>MSIKEMPFITCDEFNGVPSYMKSRLTYNQINDVIKEINKAVISKYKILHQPKKSMNSVTRNLYHRFIDEETKDTKGRYFIVEADIKEFTTLKADKKFHVLLNILRHCRRLSEVRGGGLTRYVIT[2x]

Originally discovered in a proteomics screen, the Ska complex is now recognized as a key element required for maintaining stable KT–MT attachments. The ternary Ska complex, composed of Ska1, Ska2 and Ska3, localizes to the outer KT in a KMN-dependent manner. Although GST–Ska1133–255 is not strictly equivalent to the FL Ska1 dimer in the native complex, and thus might bind MTs differently, it clearly interacted with MTs more efficiently than Ska1133–255. These observations suggest that Ska1133–255 (from now on referred to as MTBD) is the major MT-binding element within the Ska complex, which, on dimerization, can bind MTs more efficiently. Here we have used biochemical and high-resolution structural analysis to show that the human Ska complex interacts with MTs through the C-terminal domain of Ska1, which forms a variant form of winged-helix domain.

To understand the structural basis for the ability of human Ska complex to bind MTs, we obtained crystals of the Ska1–MTBD in two different crystal forms that diffracted X-rays to about 2 Å. Models from crystal form I (space group C2221) and II (space group P32) were refined to 2.1 and 2.3 Å with R factors of 19.6 and 22.5, and Rfree factors of 25.1 and 26.8, respectively, and superpose well with an overall root mean square deviation of 0.6 Å. Residues 133–142 are stabilized in an extended conformation, followed by eight α-helical segments (α1–α8) and a C-terminal β-hairpin. The structural analysis showed that the Ska1–MTBD is related to a winged-helix domain, a domain known for its ability to bind DNA and in mediating protein–protein interactions. The Ska1–MTBD differs from the canonical winged-helix domain by the incorporation of two additional modules. Analysis of the electrostatic surface potential revealed the existence of contiguous positively charged patches all over the Ska1–MTBD surface, suggesting the potential involvement of multiple MT contact sites. Although mutations at K170/177 and K135/203/206 showed no major effects on MT binding, mutations at R155/236/245, a region reported recently to be critical for MT binding, together with two new regions identified in this study, K183/184/203/206 and K217/223/226/227, all showed significant reductions in MT binding (Kd=20±4.5, 17.1±5.5 and 14.5±2.8 μM, respectively, versus WT=2.9±0.6 μM), pointing to the existence of multiple MT interaction sites. Confirming this notion, a combination of R236/245A with R155A resulted in stronger reduction in MT binding than R236/245A alone, and the simultaneous mutation of multiple clusters (K183/184/203/206/217/223/226/227/R236/245A) almost completely abolished MT binding. These results provide clear evidence that the human Ska complex binds MTs through a multipartite binding mode of Ska1–MTBD. Remarkably, the tubulin contact sites are dispersed across the surface of the Ska1–MTBD and distances between different contact sites range between 15 and 30 Å.>GGGGCCGGGGCC[6x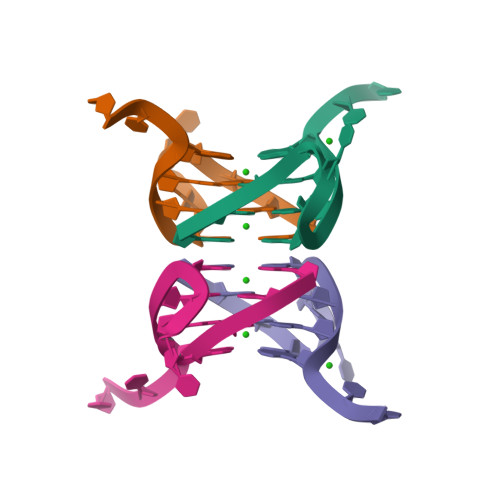]N-(2-chlorophenyl)-N-methyl-4H-thieno[3,2-c]chromene-2-carboxamide 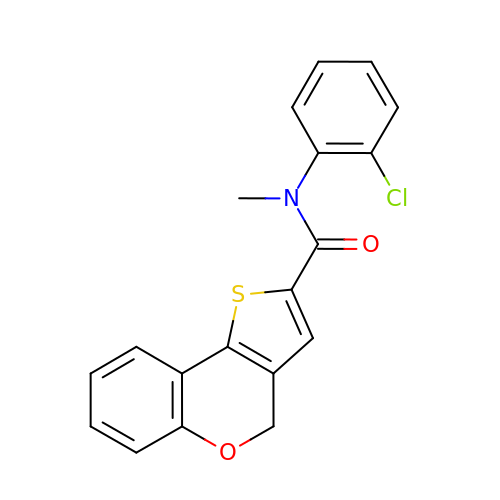| C19 H14 Cl N O2 S | PCSYEOAUKWBYOX-UHFFFAOYSA-N2'-MONOPHOSPHOADENOSINE-5'-DIPHOSPHORIBOSE | C15 H29 N5 O17 P3 | 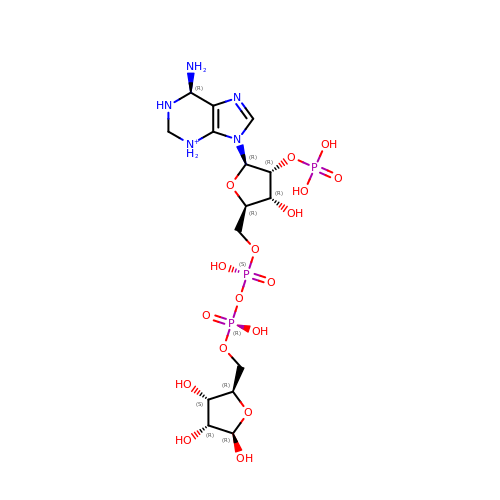QHNQLFGTVLWISK-MQSGHBOVSA-O> MSLSLFGVKNNWHKNGIWWFSKILNKTVGEERYDALRVQRRIWSMRFYYARQQCLYELFVDHPDLAQWTGTYPKVDSSHGFPFYSTYEMYRDFQENTLNSDGS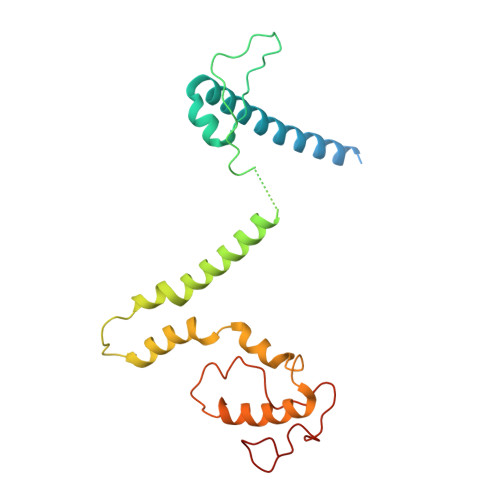FAQWITLVCGIYVIHVIYNYMIPYYWVSTPLKNDEFTRLRMKDYIASTVLEEVYGISYAEWGWLPHDFAYNRMRGLAGYMHPDDPRAMCTSTFHRKHKYIEHEVEKVGDYHHMTYPK> MVAASEGNVVIEVDMANGWRGNASGSTSHSGITYSADGVTFAALGDGVGAVFDIARPTTLEDAVIAMVVNVSAEFKASEANLQIFAQLKEDWSKGEWDCLAASSELTADTDLTLTCTIDEDDDKFNQTARDVQVGIQAKGTPAGTITIKSVTITLAQEAYSANVDHLRDLAPSDFPIGVAVSNTDSATYNLLTNSREQAVVKKHFNHLTAGNIMKMSYMQPTEGNFNFTNADAFVDWATENNMTVHGHALVWHSDYQVPNFMKNWAGSAEDFLAALDTHITTIVDHYEAKGNLVSWDVVNEAIDDNSPANFRTTDSAFYVKSGNSSVYIERAF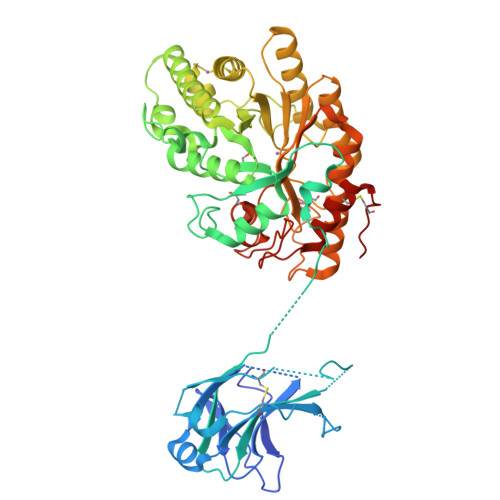QTARAADPAVILYYNDYNIEQNNAKTTKMVDMVKDFQARSIPIDGVGFQMHVCMNYPSIANISAAMKKVVDLGLLVKITELDVAVNQPHCDAYPANKINPLTEAAQLAQKKRYCDVVKAYLDTVPVNQRGGISVWGTTDANTWLDGLYREQFEDEKISWPLLFDNNYNDKPALRGFADALIGTQCTNTHELHHHHHH Glutamine synthetase (GS) plays a crucial role in nitrogen metabolism by catalyzing the ATP-dependent condensation of glutamate with ammonia to produce glutamine, ADP, and inorganic phosphate. Drosophila melanogaster GS (DmGS) has two forms, namely, isoform I (DmGS1) and isoform II (DmGS2). The cytoplasmic DmGS2 is the most abundant form in adult flies, comprising 90% of total GS activity. The three-dimensional structure of eukaryotic GS has revealed a decamer consisting of two stacked pentamers.

Herein, we report the X-ray crystallographic structure of DmGS2 in the ADP-bound state. Within the decameric structure of DmGS2, each monomer bound ADP with identical protein-ADP interactions. DmGS2 had six additional N-terminal residues (NSARIL) that formed a turn not being found in other GSs. The short helices, α-1 and α-2, the so-called meander region, located in the N-terminal region of DmGS2 was highly variable and also observed in other GSs, such as human and M. tuberculosis using ConSurf analysis. Moreover, the meander region of DmGS2 made contacts with neighboring subunits in the core of the pentamer. In addition, the pentameric structure of DmGS2 indicated that Asn11 and Arg13 from one subunit made H-bonds with nearest-neighbor subunits at Val176, Ala178, and Ile 5, respectively. Arg4 in each protomer of one pentamer forms H-bonds with Glu7 and Asp8 in each monomer of the other pentamer. Furthermore, Arg 13 from one subunit forms an H-bond with Ile 5 of the neighboring subunit in the other pentamer. Those interactions in the N-terminal meander region of DmGS2 may stabilize the five monomers and strengthen pentamer–pentamer interactions compared with other GSs. Thus, R4D was sedimented as a large, random oligomer. These data indicated that the N-terminal meander region that includes R4 is essential for pentamer formation and stability.

>[10x]ARILEDSPNARINKTILDRYLSLPLQENIVQATYVWIDGTGEDLRCKDRTLDFIPQSPKELPVWNYDGSSCYQAEGSNSDTYLYPVAIYKDPFRRGNNILVMCDTYKFDGTPTDTNKRKTCLEVANKCAAEEPWFGIEQEYTFLDFDGHPLGWPKNGFPGPQGPYYCGVGANKVYARDIVDAHYRACLYAGIKVSGTNAEVMPAQWEFQVGPCEGISIGDDLWMARFLLHRISEEFGIVSTLDPKPMPGDWNGAGAHTNVSTKAMREDGGIRDIEKAVAKLSKCHERHIRAYDPKQGQDNARRLTGKHETSSINDFSAGVANRGCSIRIPRGVNDDGKGYFEDRRPSSNCDPYSVVEAILRTICLDE>MSQHNEKNPHQHQSPLHDSSEAKPGMDSLAPEDGSHRPAAEPTPPGAQPTAPGSLKAPDTRNEKLNSLEDVRKGSENYALTTNQGVRIADDQNSLRAGNRGPTLLEDFILREKITHFDHERIPERIVHARGSAAHGYFQPYKSLSDITKADFLSDPNKITPVFVRFSTVQGGAGSADTVRDIRGFATKFYTEEGIFDLVGNNTPIFFIQDAHKFPDFVHAVKPEPHWAIPQGQSAHDTFWDYVSLQPETLHNVMWAMSDRGIPRSYRTMEGFGIHTFRLINAEGKATFVRFHWKPLAGKASLVWDEAQKLTGRDPDFHRRELWEAIEAGDFPEYELGFQLIPEEDEFKFDFDLLDPTKLIPEELVPVQRVGKMVLNRNPDNFFAENEQAAFHPGHIVPGLDFTNDPLLQGRLFSYTDTQISRLGGPNFHEIPINRPTCPYHNFQRDGMHRMGIDTNPANYEPNSINDNWPRETPPGPKRGGFESYQERVEGNKVRERSPSFGEYYSHPRLFWLSQTPFEQRHIVDGFSFELSKVVRPYIRERVVDQLAHIDLTLAQAVAKNLGIELTDDQLNITPPPDVNGLKKDPSLSLYAIPDGDVKGRVVAILLNDEVRSADLLAILKALKAKGVHAKLLYSRMGEVTADDGTVLPIAATFAGAPSLTVDAVIVPCGNIADIADNGDANYYLMEAYKHLKPIALAGDARKFKATIKIADQGEEGIVEADSADGSFMD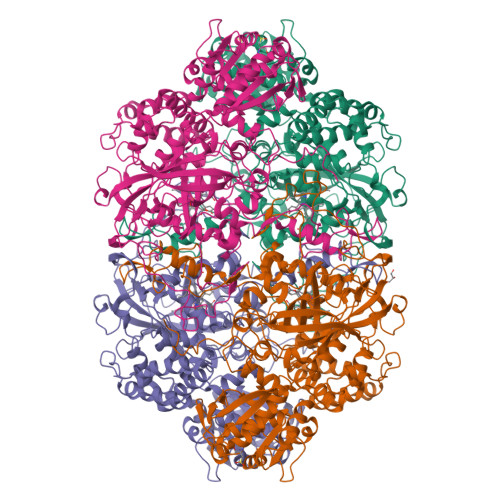ELLTLMAAHRVWSRIPKIDKIPA[4x]>MGSSHHHHHHSQDPMSLNLVSEQLLAANGLKHQDLFAILGQLAERRLDYGDLYFQSSYHESWVLEDRIIKDGSYNIDQGVGVRAISGEKTGFAYADQISLLALEQSAQAARTIVRDSGDGKVQTLGAVEHSPLYTSVDPLQSMSREEKLDILRRVDKVAREADKRVQEVTASLSGVYELILVAATDGTLAADVRPLVRLSVSVLVEEDGKRERGASGGGGRFGYEFFLADLDGEVRADAWAKEAVRMALVNLSAVAAPAGTMPVVLGAGWPGVLLHEAVGHGLEGDFNRRGTSVFSGQVGELVASELCTVVDDGTMVDRRGSVAIDDEGTPGQYNVLIENGILKGYMQDKLNARLMGMTPTGNGRRESYAHLPMPRMTNTYMLPGKSTPQEIIESVEYGIYAPNFGGGQVDITSDKFVFSTSEAYLIENGKVTKPVKGATLIGSGIETMQQISMVGNDLKLDNGVGVCGKEGQSLPVGVGQPTLKVDNLTVGGTA[2x];>[2x]MALAMKVISQVEAQRKILEEAVSTALELASGKSDGAEVAVSKTTGISVSTRYGEVENVEFNSDGALGITVYHQNRKGSASSTDLSPQAIARTVQAALDIARYTSPDPCAGVADKELLAFDAPDLDLFHPAEVSPDEAIELAARAEQAALQADKRITNTEGGSFNSHYGVKVFGNSHGMLQGYCSTRHSLSSCVIAEENGDMERDYAYTIGRAMSDLQTPEWVGADCARRTLSRLSPRKLSTMKAPVIFANEVATGLFGHLVGAIAGGSVYRKSTFLLDSLGKQILPDWLT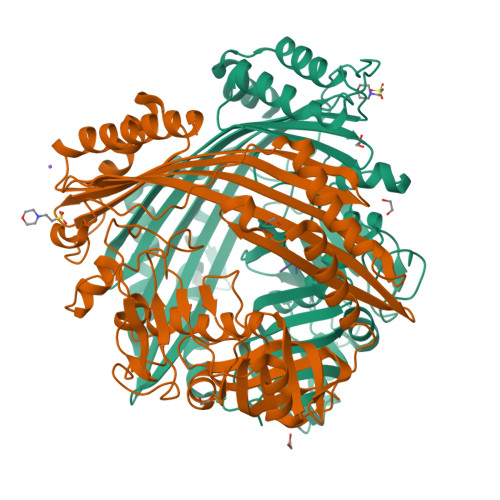IEEHPHLLKGLASTPFDSEGVRTERRDIIKDGILTQWLLTSYSARKLGLKSTGHAGGIHNWRIAGQGLSFEQMLKEMGTGLVVTELMGQGVSAITGDYSRGAAGFWVENGEIQYPVSEITIAGNLKDMWRNIVTVGNDIETRSNIQCGSVLLPEMKIAGQ;>HPF[2x]>MDKTVLDANLDPLKGKTIGVIGYGNQGRVQATIMRENGLNVIVGNVKDKYYELAKKEGFEVYEIDEAVRRSDVALLLIPDEVMKEVYEKKIAPVLQGKKEFVLDFASGYNVAFGLIRPPKSVDTIMVAPRMVGEGIMDLHKQGKGYPVLLGVKQDASGKAWDYAKAIAKGIGAIPGGIAVISSFEEEALLDLMSEHTWVPILFGAIKACY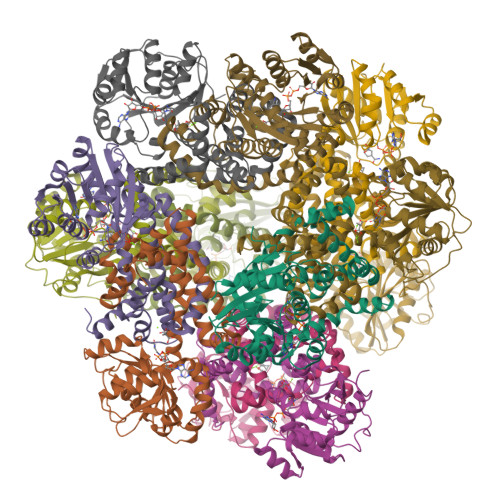DIAVKEYGVSPEAALLEFYASGELAEIARLIAEEGIFNQMVHHSTTSQYGTLTRMFKYYDVVRRIVENEAKYIWDGSFAKEWSLEQQAGYPVFYRLWELATQSEMAKAEKELYKLLGRKVKND[12x]(2R,5S)-5-[(1R)-1,2-dihydroxyethyl]-3,3,4,4-tetrafluorotetrahydrofuran-2-yl 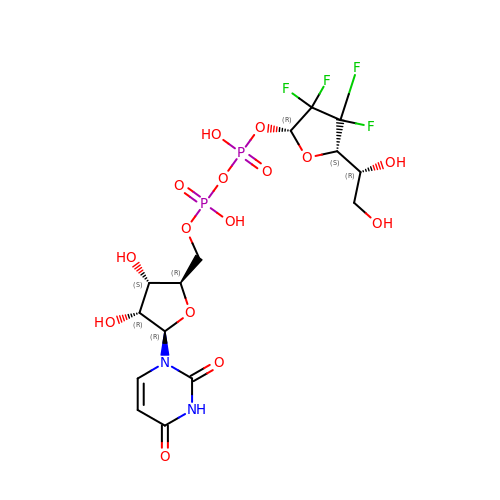[(2R,3S,4R,5R)-5-(2,4-dioxo-3,4-dihydropyrimidin-1(2H)-yl)-3,4-dihydroxytetrahydrofuran-2-yl]methyl dihydrogen diphosphate (non-preferred name) | C15 H20 F4 N2 O15 P2 | QGSSIXQRPAELEQ-UMEAPJPCSA-N1-butyl-3-(4-{[(2Z,4R)-2-imino-4-methyl-4-(2-methylpropyl)-5-oxoimidazolidin-1-yl]methyl}benzyl)urea 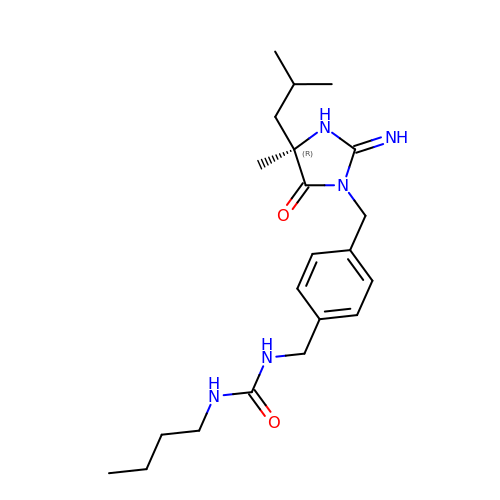| C21 H33 N5 O2 | VPGRKPRUHRVZER-OAQYLSRUSA-N>MKTIIINGVQFNTDEDTTILKFARDNNIDISALCFLNNCNNDINKCEICTVEVEGTGLVTACDTLIEDGMIINTNSDAVNEKIKSRISQLLDIHEFKCGPCNRRENCEFLKLVIKYKARASKPFLPKDKTEYVDERSKSLTVDRTKCLLCGRCVNACGKNTETYAMKFLNKNGKTIIGAEDEKCFDDT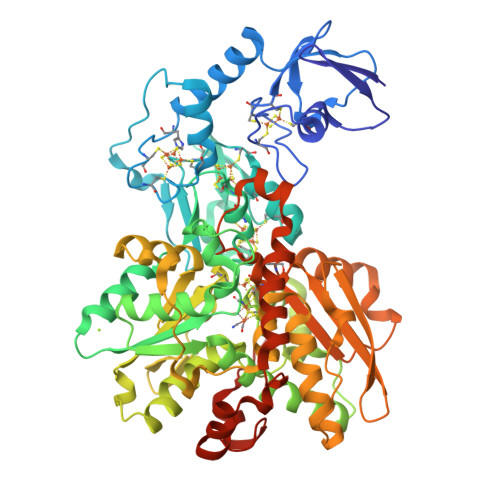NCLLCGQCIIACPVAALSEKSHMDRVKNALNAPEKHVIVAMAPSVRASIGELFNMGFGVDVTGKIYTALRQLGFDKIFDINFGADMTIMEEATELVQRIENNGPFPMFTSCCPGWVRQAENYYPELLNNLASAKSPQQIFGTASKTYYPSISGLDPKNVFTVTVMPCTSKKFEADRPQMEKDGLRDIDAVITTRELAKMIKDAKIPFAKLEDSEADPAMGEYSGAGAIFGATGGVMEAALRSAKDFAENAELEDIEYKQVRGLNGIKEAEVEINNNKYNVAVINGASNLFKFMKSGMINEKQYHFIEVMACHGGCVNGGGQPHVNPKDLEKVDIKKVRASVLYNQDEHLSKRKSHENTALVKMYQNYFGKPGEGRAHEILHFKYKKSAWSHPQFEK[2x]> MKFSELWLREWVNPAIDSDALANQITMAGLEVDGVEPVAGSFHGVVVGEVVECAQHPNADKLRVTKVNVGGDRLLDIVCGAPNCRQGLRVAVATIGAVLPGDFKIKAAKLRGEPSEGMLCSFSELGISDDHSGIIELPADAPIGTDIREYLKLDDNTIEISVTPNRADCLGIIGVARDVAVLNQLPLVQPEIVPVGATIDDTLPITVEAPEACPRYLGRVVKGINVKAPTPLWMKEKLRRCGIRSIDAVVDVTNYVLLELGQPMHAFDKDRIEGGIVVRMAKEGETLVLLDGTEAKLNADTLVIADHNKALAMGGIFGGEHSGVNDETQNVLLECAFFSPLSITGRARRHGLHTDASHRYERGVDPALQHKAMERATRLLIDICGGEAGPVIDITNEATLPKRATITLRRSKLDRLIGHHIADEQVTDILRRLGCEVTEGKDEWQAVAPSWRFDMEIEEDLVEEVARVYGYNNIPDEPVQASLIMGTHREADLSLKRVKTLLNDKGYQEVITYSFVDPKVQQMIHPGVEALLLPSPISVEMSAMRLSLWTGLLATVVYN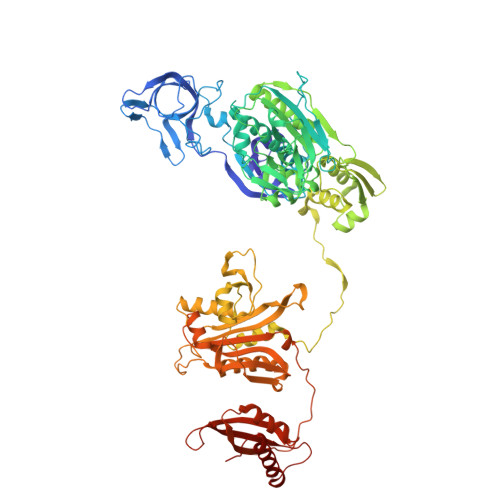QNRQQNRVRIFESGLRFVPDTQAPLGIRQDLMLAGVICGNRYEEHWNLAKETVDFYDLKGDLESVLDLTGKLNEVEFRAEANPALHPGQSAAIYLKGERIGFVGVVHPELERKLDLNGRTLVFELEWNKLADRVVPQAREISRFPANRRDIAVVVAENVPAADILSECKKVGVNQVVGVNLFDVYRGKGVAEGYKSLAISLILQDTSRTLEEEEIAATVAKCVEALKERFQASLRD>MIPGANLLRMAFGVIGTQIVKYRKFEQRVKNDQAQYVSMFEEPFDLAASVQRVRRDQYVQFNLEFQRNYVMIFANFEMVDLDRDVAGDQFLWTGRVFQLESQGSWFYQDGWGVCLAVDIGAAKLTDDGKPTF[6x];>MFDGELIAKMVVELNAAMTSAQEALQFPDFEVVQKAQPTQQGTSTRPTIFFQKLFDIPRGWPATDWHLDNTTRKYVEITRQHVETTFQISSLHWQNPEITHVVTASDIANYVRAYFQARSTIERVKELDFLILRVSQISNEAFENDNHQFEFHPSFDMVVTYNQYIRLYENAAYSADGVLIGV[6x];>MINISAFGSICQFTASRTFPNGFTVTEFADDADPIDSPPFTAADTGVGLNGDMVVWNRANILEVVVNVIPNTEGERNLAVLLDANRTGKDKSGARDVVGLVVAMPDGSKITCTNGTPIDGVLINAVASVGRLKTKPYRFRFEKVIKAGTS[6x];> MISQSRYIRIISGVGAGAPVAGRKLILRVMTTNNVIPPGIVIEFDNSNAVMSYFGAQSEEYQRAAAYFKFISKSVNSPSSISFARWVNTAIAPMVVGDNLPKTIADFAGFSAGVLTIMVGAAEKNITAIDTSAATSMDNVASIIQTEIRKNTDPQLAQATVTWNQNTNQFTLVGATIGTGVLAVAKSADPQDMSTALGWSTSNVVNVAGQAADLPDAAVAKSTNVS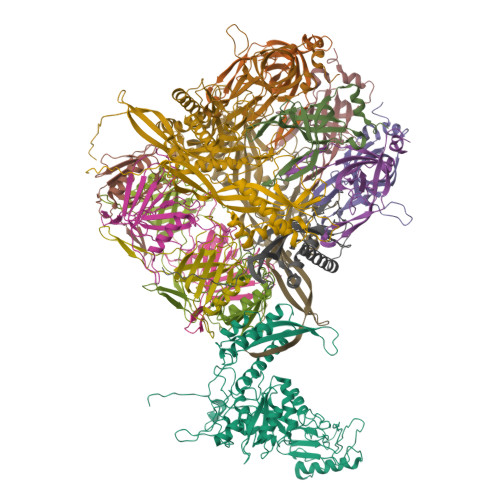NNFGSFLFAGAPLDNDQIKAVSAWNAAQNNQFIYTVATSLANLGTLFDLVKGNAGTGLHVLSATAANDFVEQCPSEIFAATNYDEPGASQNYMYYQFPGRNITVSDDTVANTVDKSRGNYIGVTQANGQQLAFYQRGILCGGPTDAVDMNVYANEIWLKSAIAQALLDLFLNVNAVPASSTGEAMVLAVLQPVLDKATANGTFTYGKEISAVQQQYITQVTGDRRAWRQVQTLGYWINITFSSYTNNNTGLIEWKANYTLIYSKGDAIRFVEGSDVMI>[2x]MLVLFFPLLLTVGLSTAGHVKCPDFGDWKPWTDCLWYPPQHMYSKLSHACGMHAHRNLTGVMDLPHGHKTPPPCGHCSFKFRCRRRPNTEGCYPLDGEVEVCHDHSDICTLPKLPHLGCGYAFINEKLKQCFTRPDTPSYVRLGYRKMFESIPKKHCIEKDGMCKCCCGDYEPNESG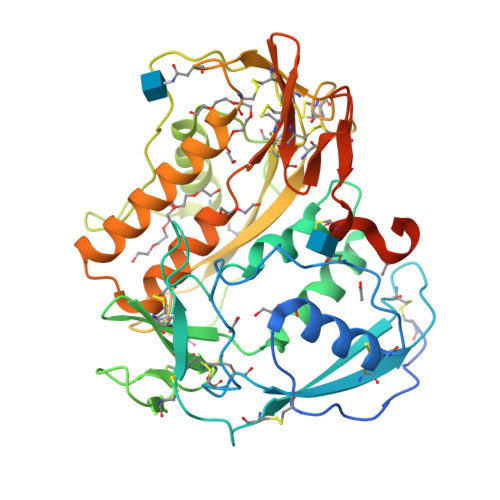TECIKPPAHDCPAYGPPSEWSECLWFPLKNIVSHVYDHCHVHKEPDGYEPHSVAPANVHIPEKCGFCSFRVKCMKRDKKDGCFPLKLGKKSCGKDDCPTCGDICTLDKINGSCAFPRVMKEKIWDDFTATSKEKHMPHWKRDGYAKMLMQLPYSNCKEVGDKCKCCCHPYEPNKDGTACVVKEYCKRVHELHHHDHHGHGEEHHKSSSSESKEHHHH>[3x]TFFKTVYR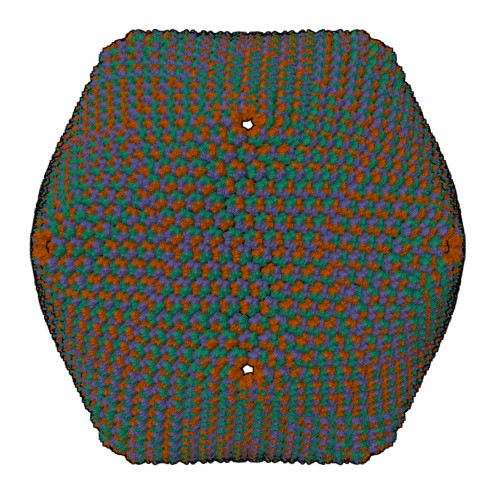RYTNFAIESIQQTINGSVGFGNKVSTQISRNGDLITDIVVEFVLTKGGNGGTTYYPAEELLQDVELEIGGQRIDKHYNDWFRTYDALFRMNDDRYNYRRMTDWVNNELVGAQKRFYVPLIFFFNQTPGLALPLIALQYHEVKLYFTLASQVQGVNYNGSSAIAGAAQPTMSVWVDYIFLDTQERTRFAQLPHEYLIEQLQFTGSETATPSATTQAAQNIRLNFNHPTKYLAWNFNNPTNYGQYTALANIPGACSGAGTAAATVTTPDYGNTGTYNEQLAVLDSAKIQLNGQDRFATRKGSYFNKVQPYQSIGGVTPAGVYLYSFALKPAGRQPSGTCNFSRIDNATLSLTYKTCSIDATSPAAVLGNTETVTANTATLLTALNIYAKNYNVLRIMSGMGGLAYAN> MGSSHHHHHHSSGLENLYFQGSDQVQKVDQYLYHMRLSDETLLEISKRFRKEMEKGLGATTHPTAAVKMLPTFVRSTPDGTEHGEFLALDLGGTNFRVLWVKVTDNGLQKVEMENQIYAIPEDIMRGSGTQLFDHIAECLANFMDKLQIKDKKLPLGFTFSFPCHQTKLDESFLVSWTKGFKSSGVEGRDVVALIRKAIQRRGDFDIDIVAVVNDTVGTMMTCGYDDHNCEIGLIVGTGSNACYMEEMRHIDMVEGDEGRMCINMEWGAFGDDGSLNDIRTEFDQEIDMGSLNPGKQLFEKMISGMYMGELVRLILVKMAKEELLFGGKLSPELLNTGRFETKDISDIEGEKDGIRKAREVLMRLGLDPTQEDCVATHRICQIVSTRSASLCAATLAAVLQRIKENKGEERLRSTIGVDGSVYKKHPHFAKRLHKTVRRLVPGCDVRFLRSEDGSGKGAAMVTAVAYRLADQHRARQKTLEHLQLSHDQLLEVKRRMKVEMERGLSKETHASAPVKMLPTYVCATPDGTEKGDFLALDLGGTNFRVLLVR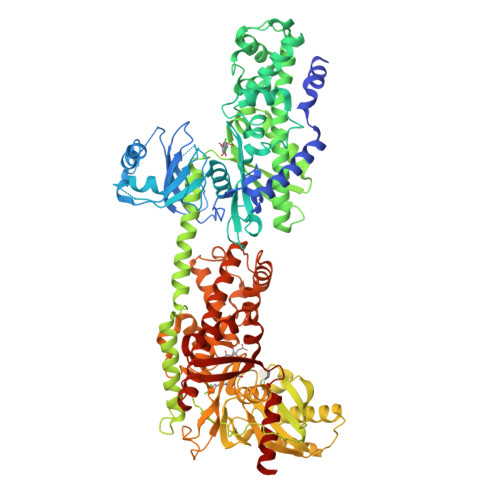VRNGKWGGVEMHNKIYAIPQEVMHGTGDELFDHIVQCIADFLEYMGMKGVSLPLGFTFSFPCQQNSLDESILLKWTKGFKASGCEGEDVVTLLKEAIHRREEFDLDVVAVVNDTVGTMMTCGFEDPHCEVGLIVGTGSNACYMEEMRNVELVEGEEGRMCVNMEWGAFGDNGCLDDFRTEFDVAVDELSLNPGKQRFEKMISGMYLGEIVRNILIDFTKRGLLFRGRISERLKTRGIFETKFLSQIESDCLALLQVRAILQHLGLESTCDDSIIVKEVCTVVARRAAQLCGAGMAAVVDRIRENRGLDALKVTVGVDGTLYKLHPHFAKVMHETVKDLAPKCDVSFLQSEDGSGKGAALITAVACRIREAGQ>ADLNTEGDALYSLRQSLKDANNVLQSWDPTLVNPCTWFHVTCNPDNSVIRVDLGNAQLSGALVPQLGQLKNLQYLELYSNNISGTIPNELGNLTNLVSLDLYLNNFTGFIPETLGQLYKLRFLRLNNNSLSGSIPKSLTNITTLQELALDTNQLKSVPDGIFDRLTSLQKIWLHTNPWDCSCPRIDYLSRWLNKNSQKEQGSAKCSGSGKPVRSIICPTSAS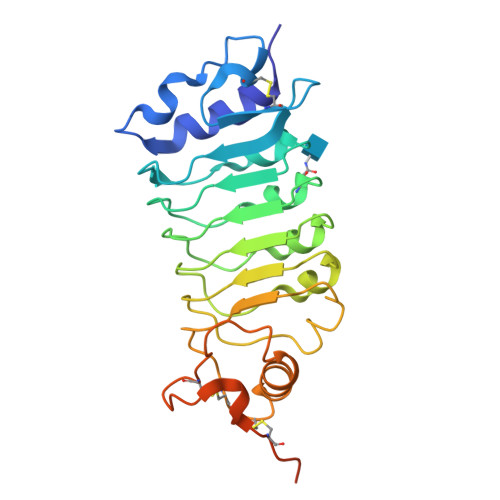LVPRGSWSHPQFEKGSHHHHHH[2x]> MQSSTSTDQHVLHHMDPHRFTSQIPTATSSQLRRRNSTNQGLTDMINKSIARNTISGTGIPTGGINKNKRTRSTVAGGTNGTALALNDKSNSRNSVSRLSINQLGSLQQHLSNRDPRPLRDKNFQSAIQEEIYDYLKKNKFDIETNHPISIKFLKQPTQKGFIIIFKWLYLRLDPGYGFTKSIENEIYQILKNLRYPFLESINKSQISAVGGSNWHKFLGMLHWMVRTNIKLDMCLNKVDRSLINQNTQEITILSQPLKTLDEQDQRQERYELMVEKLLIDYFTESYKSFLKLEDNYEPSMQELKLGFEKFVHIINTDIANLQTQNDNLYEKYQEVMKISQKIKTTREKWKALKSDSNKYENYVNAMKQKSQEWPGKLEKMKSECELKEEEIKALQSNISELHKILRKKGISTEQFELQNQEREKLTRELDKINIQSDKLTSSIKSRKLEAEGIFKSLLDTLRQYDSSIQNLTRSRSQLGHNVNDSSLKINISENLLDRDFHEGISYEQLFPKGSGINESIKKSILKLNDEIQERIKTIEKDNITL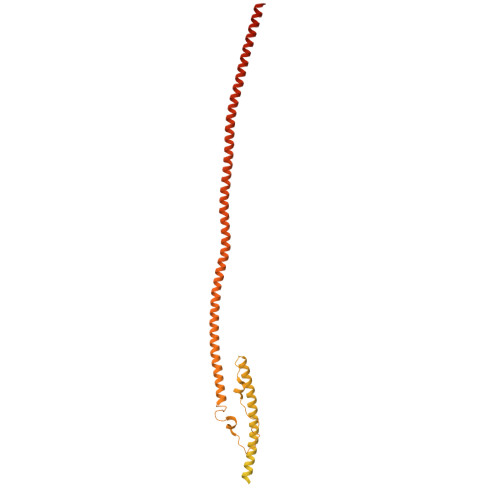EKDIKNLKHDINEKTQINEKLELELSEANSKFELSKQENERLLVAQRIEIEKMEKKINDSNLLMKTKISDAEELVTSTELKLEELKVDLNRKRYKLHQQVIHVIDITSKFKINIQSSLENSENELGNVIEELRNLEFETEHNVTN>QQNLPQRYIELVVVADHRVFM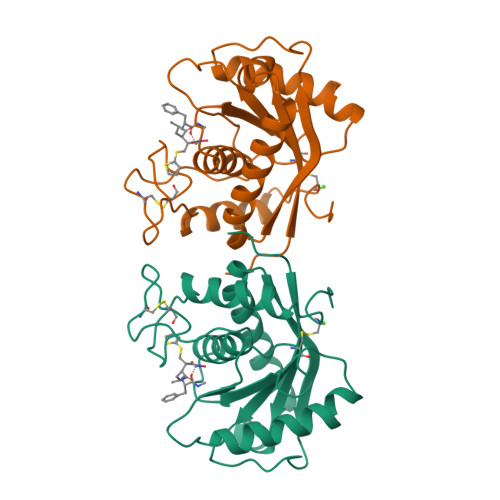KYNSDLNTIRTRVHEIVNFINGFYRSLNIHVSLTDLEIWSNEDQINIQSASSDTLNAFAEWRETDLLNRKSHDNAQLLTAIELDEETLGLAPLGTMCDPKLSIGIVQDHSPINLLMGVTMAHELGHNLGMEHDGKDCLRGASLCIMRPGLTKGRSYEFSDDSMHYYERFLKQYKPQCILNKP[2x]>YPESIDWREKGAVTPVKNQNPCGSCWAFSTVATIEGINKIITGQLISLSEQELLDCERRSHGCDGGYQTTSLQYVVDNGVHTEREYPYEKKQGRCRAKDKKGPKVYITGYKYVPANDEISLIQAIANQPVSVVTDSRGRGFQFYKGGIYEGPCGTNTDHAVTAVGYGKTYLLLKNSWGPNWGEKGYIRIKRASGRSKGTCGVYTSSFFP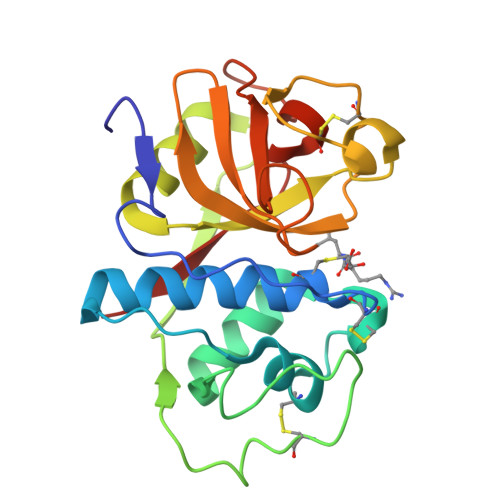IKGYR[4x]>KHSLPDLPYDYGALEPHIN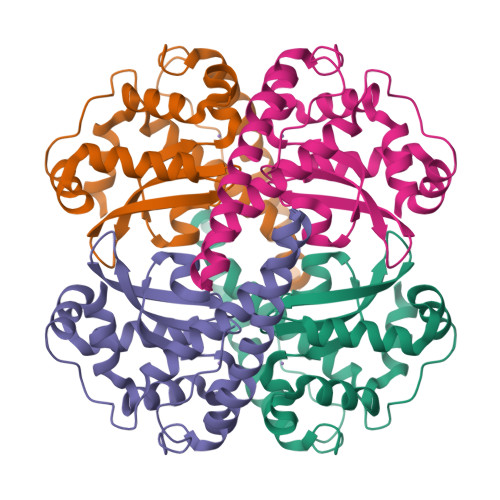AQIMQLHHSKHHAAYVNNLNVTEEKYQEALAKGDVTAQIALQPALKLNGGGHINHSIFWTNLSPNGGGEPKGELLEAIKRDFGSFDKFKEKLTAASVGVQGSGWGWLGFNKERGHLQIAACPNQDPLQGTTGLIPLLGIDVWEHAYYLQYKNVRPDYLKAIWNVINWENVTERYMAC[2x]(S)-2-(4-chlorophenyl)-2-pyridin-3-yl-1-[4-[4-(trifluoromethyl)phenyl]piperazin-1-yl]ethanone | C24 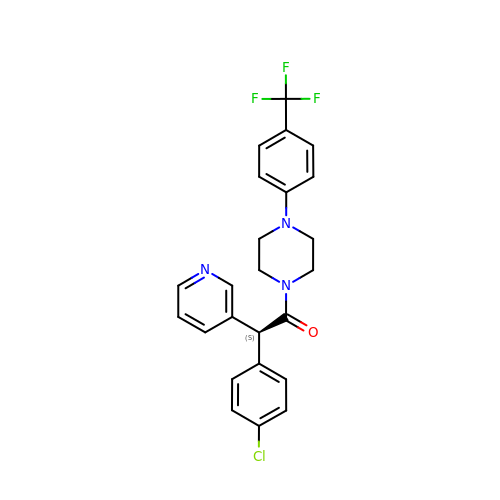H21 Cl F3 N3 O | OJFZYAQGMWSUID-QFIPXVFZSA-N> KETAAAK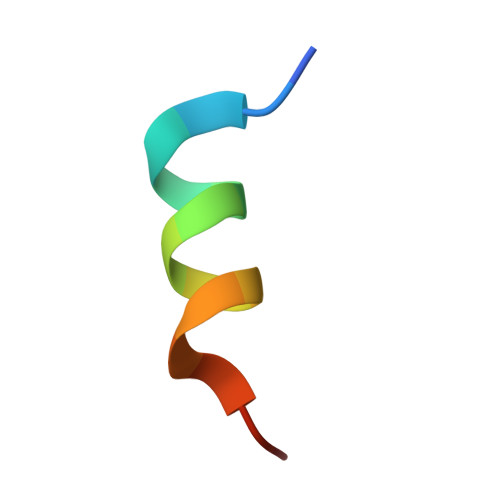FERQHGDSX> MRLVLEEPFKRLWNGRDPFEAVEALQGKVYRELEGRRTLRTEVDGRGYFVKIHRGIGWGEIAKNLLTAKLPVLGARQEWQAIRRLHEAGVATMTAVAYGERGSDPARQHSFIVTEELAPTVDLEVFSQDWRERPPPPRLKRALVEAVARMVGDMHRAGVNHRDCYICHFLLHTDKPVSADDFRLSVIDLHRAQTRDATPKRWRNKDLAALYFSALDIGLTRRDKLRFLRTYFRRPLREILRDEAGLLAWMERKAEKLYE;> TIEERVKKIIGEQLGVKQEEVT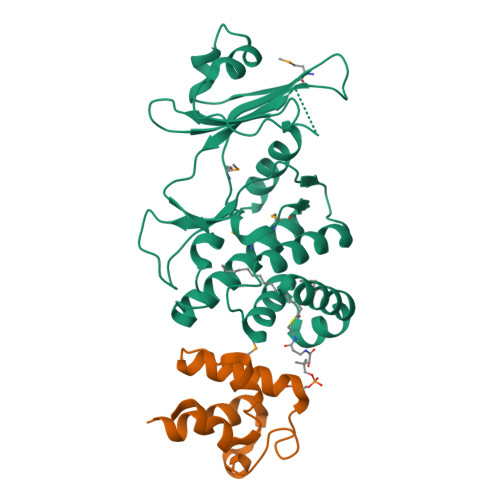NNASFVEDLGADSLDTVELVMALEEEFDTEIPDEEAEKITTVQAAIDYIN>APQLHHHHHHDLYENLYFQGKLDPASKSRSCGEVRQIYGAKGFSLSDVPQAEISGEHLRICPQGYTCCTSEMEENLANRSHAELETALRDSSRVLQAMLATQLRSFDDHFQHLLNDSERTLQATFPGAFGELYTQNARAFRDLYSELRLYYRGANLHLEETLAEFWARLLERLFKQLHPQLLLPDDYLDCLGKQAEALRPFGEAPRELRLRATRAFVAARSFVQGLGVASDVVRKVAQVPLGPECSRAVMKLVYCAHCLGVPGARPCPDYCRNVLKGCLANQADLDAEWRNLLDSMVLITDKFWGTSGVESVIGSVHTWLAEAINALQDNRDTLTAKVIQGCGNPKVNPQGPGPEEKRRRGKLAPRERPPSGTLEKLVSEAKAQLRDVQDFWISLPGTLCSEKMALSTASDDRC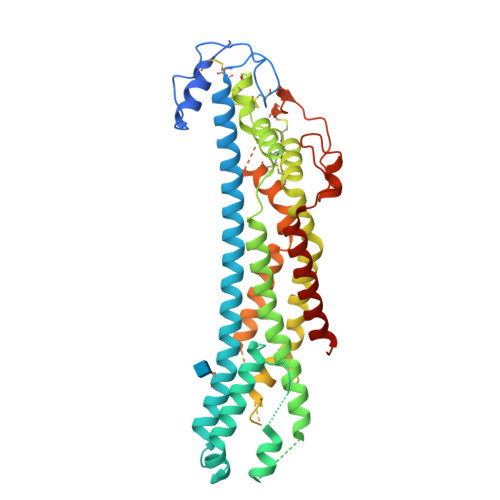WNGMARGRYLPEVMGDGLANQINNPEVEVDITKPDMTIRQQIMQLKIMTNRLRSAYNGNDVDFQ[4x]> MYVFRFHISSFHSFLVNFLQPSRGVGEPSRLLXHLETHPSYMRRVTSTAVHRTVSSVLSXALLPSFNGTLLLSVCFASCSAAPVRNLYKRLGLDHKATSEEVKAAYRQRALECHPDVVDDNQKAQAEVDFRAVSEAYDVLIDPQKRKEH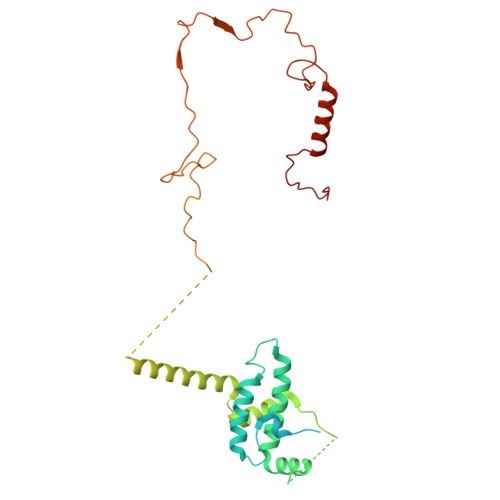DKALGLERTVPPAKKQQEGEGVGCDSKGSFNRGVTRPRNRKPFVRGDADRNFREAFHGMSLDQVLFRERLRQRRMQKQMEEKAKEGDDGSPAGREESIRRVAAAAAERFAEKVRRQYGPGMLRHARVYTSLSRDPQPPPSDYMPFRPFHGWTVPNGVRTPPEPTLGPTAKVEDVKDVQLAEPAVGDASHQRKLPKHFPVVQASDGSSLLREETIACMERERRLPHNMGKLYSYHRPY4-bromanylbenzenecarboximidamide | C7 H7 Br N2 | 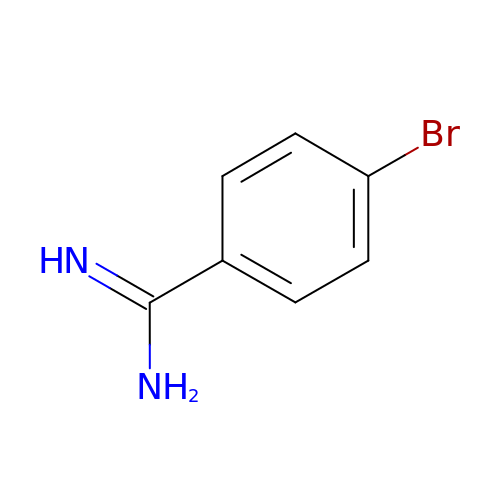JODFDXUBCBQKNC-UHFFFAOYSA-N N,N'-[ethane-1,2-diylbis(oxybenzene-3,1-diyl)]dithiophene-2-carboximidamide | 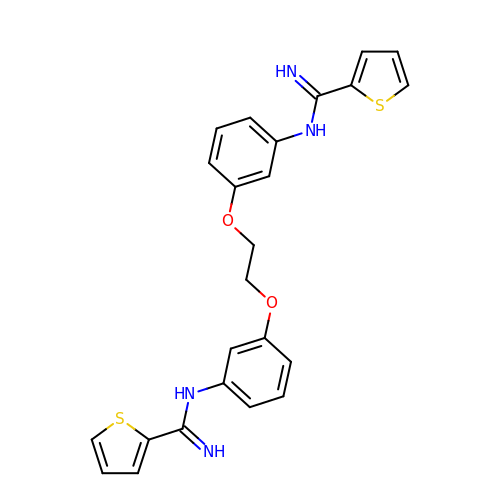C24 H22 N4 O2 S2 | FJVFGYSUSVNZDG-UHFFFAOYSA-N(4-azanylbutylamino)methanediol | C5 H14 N2 O2 | 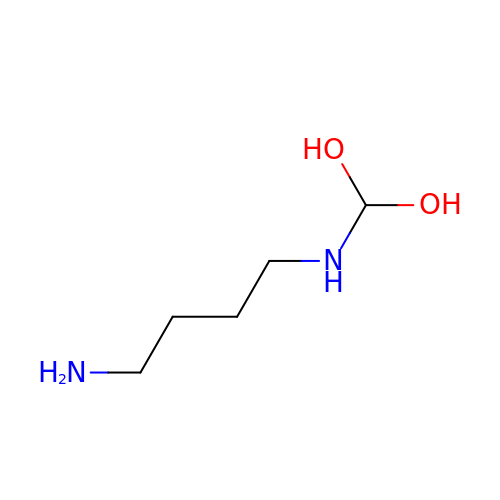JXQFUOSMIWOVKO-UHFFFAOYSA-N> MRGSHHHHHHGSSVFHNWLLEIACENYFVYIKRLSANDTGATGGHQVGLYIPSGIVEKLFPSINHTRELNPSVFLTAHVSSHDCPDSEARAIYYNSRHFGKTRNEKRITRWGRGSPLQDP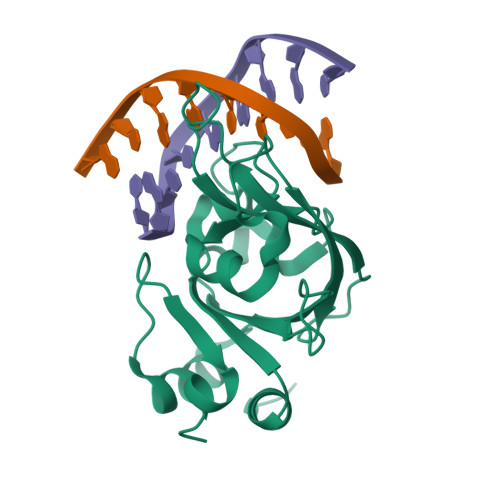ENTGALTLLAFKLDEQGGDCKEVNIWVCASTDEEDVIETAIGEVIPGALISGPAGQILGGL>[4x]GPGSMKDDHKAQHRFAGLATRAIHSGYRPDPATGAVNAPIYASSTFAQDGVGGLRGGYEYARTGNPTRTALEAALAAVEDAAFGRAFSSGMAAADCALRAMLRPGDHVVIPDDAYGGTFRLIDKVFTGWNVEYTPVALADLDAVRAAIRPTTRLIWVETPTNPLLSIADIAGIAQLGADSSAKVLVDNTFASPALQQPLSLGADVVLHSTTKYIGGHSDVVGGALVTNDEELDQSFAFLQNGAGAVPGPFDAYLTMRGLKTLVLRMQRHSENAAAVAEFLAEHPAISTVLYPGLPSHPGHAVAARQMRGFGGMVSVRMRAGRTAAEQLCAKTNIFILAESLGSVESLIEHPSAMTHASTAGSQLEVPDDLVRLSVGIEDVADLLDDLKQALG

CGS is a transferase and acts in the committed step (the fifth overall) of the biosynthesis of l-methionine. MetB is covalently linked to the cofactor pyridoxal phosphate (PLP), similar to other members of the aspartate aminotransferase (AAT-I) superfamily of enzymes. Similar to other CGS enzymes, MetB forms a homotetramer, with each individual homodimer creating two active sites. Here, we present two structures of the cystathionine γ-synthase MetB from M. ulcerans covalently linked to PLP and bound to the buffer molecule HEPES.

The crystal structure of CGS from M. ulcerans is presented covalently linked to the cofactor pyridoxal phosphate (PLP). Covalently bound at the intersection between the two monomers is the PLP-Lys208 moiety. PLP binds tightly to Lys208 with a covalent-bond length ranging between 1.3 and 1.4 Å. A similar series of sulfates are found in the MetB–PLP structure; however, there is no evidence for the presence of HEPES or any other ligand bound in the four active sites. The only noted change is seen in a loop consisting of residues 350–362, in which the disordered loop in the MetB–PLP structure becomes partially ordered in the MetB–PLP–HEPES structure. 4-succinyl-l-homoserine, l-cysteine, l-cystathionine, succinate and combinations of products and reactants proved unsuccessful, showing only the presence of the PLP covalently bound in the active site.> MAEVRQLQPDLVYGDVLVTAFINKIMRDGKKNLAARIFYDACKIIQEKTGQEPLKVFKQAVENVKPRMEVRSRRVGGANYQVPMEVSPRRQQSLALRWLVQAANQRPERRAAVRIAHELMDAA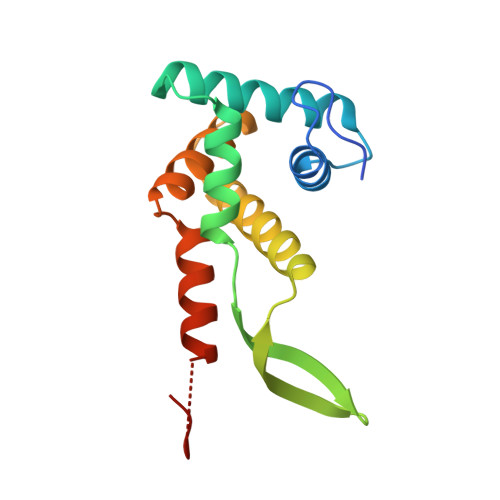EGKGGAVKKKEDVERMAEANRAYAHYRW N~2~-[4-(aminomethyl)benzyl]-N~2~-[(4-fluoro-3-methylphenyl)sulfonyl]-N-hydroxy-D-alaninamide | C18 H22 F N3 O4 S | 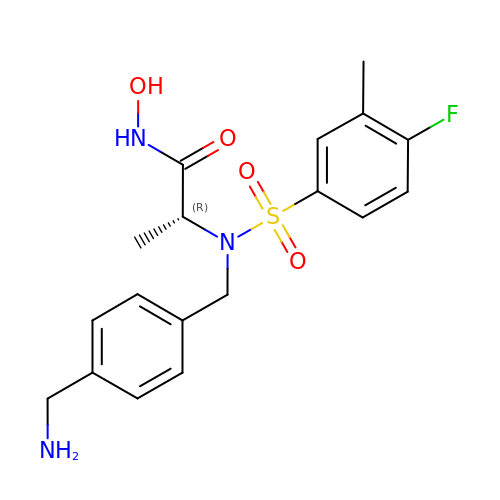CWTKLEFNKQTFGU-CYBMUJFWSA-N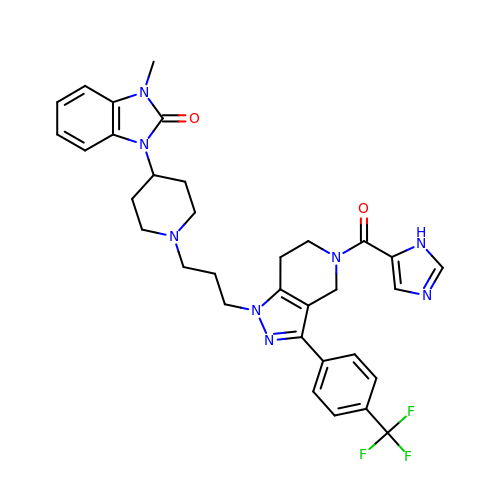1-[1-(3-{5-(1H-imidazole-5-carbonyl)-3-[4-(trifluoromethyl)phenyl]-4,5,6,7-tetrahydro-1H-pyrazolo[4,3-c]pyridin-1-yl}propyl)piperidin-4-yl]-3-methyl-1,3-dihydro-2H-benzimidazol-2-one | C33 H35 F3 N8 O2 | MHNXUUQVKHVSPU-UHFFFAOYSA-N> SVVIVGKISFCPKDVLGHGAEGTIVYRGMFDNRDVAVKRILPECFSFADREVQLLRESDEHPNVIRYFCTEKDRQFQYIAIELCAATLQEYVEQKDFAHLGLEPITLLQQTTSGLAHLHSLNIVHRDLKPHNILISMPNAHGKIKAMISDFGLCKKLAVGRHSFSRRSGVPGTEGWIAPEMLSEDCKENPTYTVDIFSAGCVFYYVISEGSHPFGKSLQRQANILLGACSLDCLHPEKHEDVIARELIEKMIAMDPQKRPSAKHVLKHPFFWSLEKQLQFF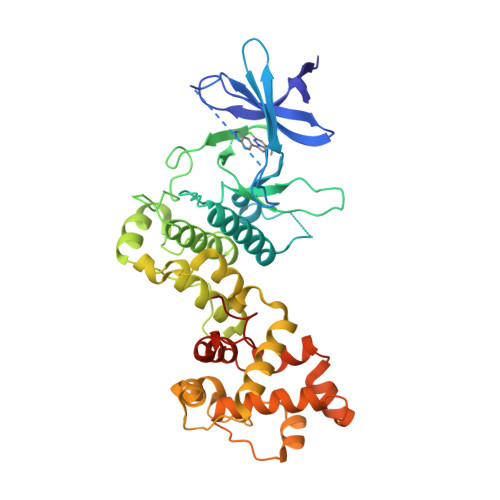QDVSDRIEKESLDGPIVKQLERGGRAVVKMDWRENITVPLQTDLRKFRTYKGGSVRDLLRAMRNKKHHYRELPAEVRETLGSLPDDFVCYFTSRFPHLLAHTYRAMELCSHERLFQPYYFHEPPEPQPPVTPDAL> MFENITAAPADPILGLADLFRADERPGKINLGIGVYKDETGKTPVLTSVKKAEQYLLENETTKN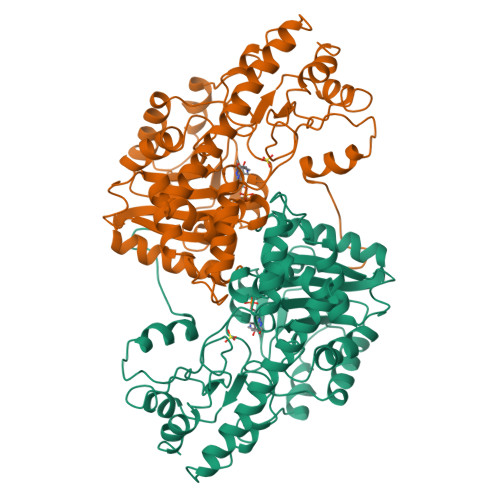YLGIDGIPEFGRCTQELLFGKGSALINDKRARTAQTPGGTGALRVAADFLAKNTSVKRVWVSNPSWPNHKSVFNSAGLEVREYAYYDAENHTLDFDALINSLNEAQAGDVVLFHGCCHNPTGIDPTLEQWQTLAQLSVEKGWLPLFDFAFQGFARGLEEDAEGLRAFAAMHKELIVASSYSKNFGLYNERVGACTLVAADSETVDRAFSQMKAAIRANYSNPPAHGASVVATILSNDALRAIWEQELTDMRQRIQRMRQLFVNTLQEKGANRDFSFIIKQNGMFSFSGLTKEQVLRLREEFGVYAVASGRVNVAGMTPDNMAPLCEAIVAVL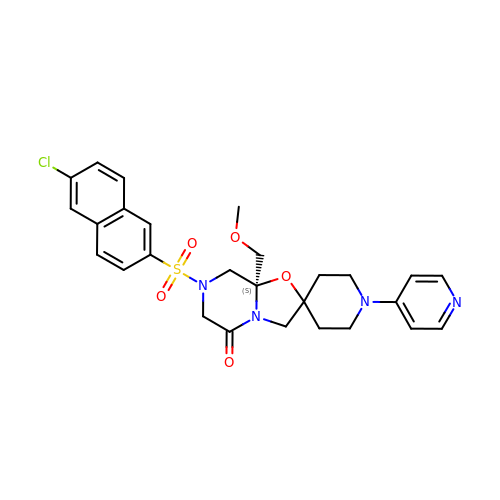(-)-7-[(6-CHLORO-2-NAPHTHALENYL)SULFONYL]TETRAHYDRO-8A-(METHOXYMETHYL)-1'-(4-PYRIDINYL)-SPIRO[5H-OXAZOLO[3,2-A]PYRAZINE-2(3H),4'-PIPERIDIN]-5-ONE | C27 H29 Cl N4 O5 S | OCCGRNQFQCNISA-MHZLTWQESA-N> SDLPPVAKAAQVVNQTLQLDDSYPDLDSYCRPGASSDYEMQSSDSSWAPFHVVRHHNIPDKVFEHLNAGEVFTKLGLFAEIGYAWASIDSSLFLWDYTHPNPELIGYEEATHTITAVALVPPKPGVFVKTITHVLVVATTSEIILLGVSATPTPSGSKSLTLYSTRMSVHRGGSDVSFIVGTKDGRIFLGGESDTDIHEIFYQQEERWFSSRCGKINHSHPFGSRQQEWLRGLYVDDTRNLLYSLSNRSTIRTYHMEGPEKLTKVIEKDKTSCLRDFAHMADSSPLFTDKTNIVALSPIPATEASKLHLMALTDTGCRLFLSATSSASYTMGGATSLAPQSMQLQFVKFPPRESPTRIRTLNGQIIDSQLDKTSRALDPSALGFRFSPGYFFDVVRKHPNQDMLFVSAPDTGRIKVTQPASALKYFEQGTWIELENGNRTI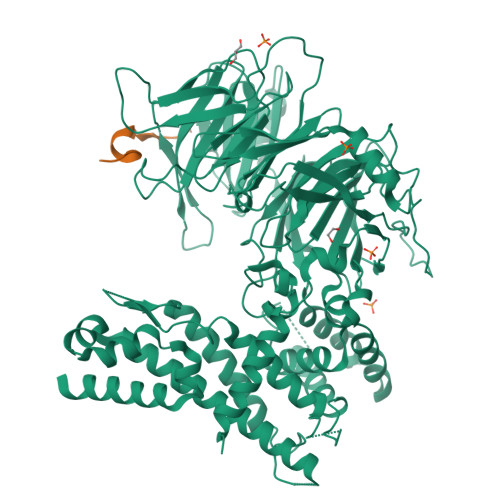EIGLTTAPFAAAKQPLGFGNELAVQFDQVPGEFAVLTNTGVHIVRRRRLVDIFAKALGNCVSASDDALEREVRKFINQYGRVETIAAALAVACGQGSDLRTGTGRGMDRNTENLARAAFIEYGGQPRLAESDGKQSVSESVRLSSRHDALALYLTRLVRTLWKAKVVQVGSGSDISSTIPTSKLVTIQENVERLRNFLEANKSTIQGLAPPSERLFGRQEDIANQKEHQALHALQKLMESISEGISFVLMLFDERVSDIYARLDAVSQQQLKDLTYEQLFSQTPGKELAKVLVKAIVNRNI;> SQDDEFCRVIPTVRKAKLLPMEEALLPAPTFTQ Stimulator of interferon genes (STING) is an antiviral signalling protein that is broadly conserved in both innate immunity in animals and phage defence in prokaryotes. Here we use cryogenic electron microscopy to determine the structure of the active Toll/interleukin-1 receptor (TIR)–STING filament complex from a Sphingobacterium faecium cyclic-oligonucleotide-based antiphage signalling system (CBASS) defence operon. To define the molecular basis of STING filament formation, we reconstituted signalling of the S. faecium TIR–STING (SfSTING) antiphage effector in vitro and used single-particle cryo-EM to determine the structure of the activated complex. In each SfSTING dimer unit, the canonical V-shaped STING CBD is positioned above two TIR enzymatic NADase domains that dock against the base of the receptor.

The partially closed 3′,3′-cGAMP-bound SfSTING conformation allows incomplete oligomerization and is incompatible with stable filamentous packing beyond about 4–6 units (or about 20 nm). Compared to the fully active SfSTING–c-di-GMP filament structure, 3′,3′-cGAMP recognition induces partial closure of the lid domain and an overall conformation of the STING CDN-binding domain (CBD) that probably weakens contact sites observed for c-di-GMP-induced filaments. Additionally, a lack of well-defined density for the TIR domains in the 3′,3′-cGAMP filaments suggests conformational flexibility that may impact stability of the filaments. Our previous results demonstrate that 3′,3′-cGAMP binds with slightly weaker affinity (about 700 nM Kd) and is unable to induce robust TIR NADase activity, findings that are now explained by our cryo-EM analysis. Compared with the modelled open apo state and partially closed 3′,3′-cGAMP-bound conformations, recognition of the signal from the correct nucleotide, c-di-GMP, induces an inward rotation of the SfSTING β-strand ‘lid’ region of about 25° and about 9° respectively and results in formation of a tightly closed complex.

>MHHHHHHGSKKRIFIGSSSEQLTILNEIVDLLGDDVECIPWTDAFALNKSGLDSLIKQTRLADYSILIATKDDLTKQRGESLTKPRDNVVFEFGLFLGAAGPEKCYLIAEEDTDLPTDLDGITVAKFTRNSGQYNSLDKIVESIRTHLVKIAEMSQLGLLPSTALAIGYYNSFIKRVCEEIHGSECVELEGKKIKVKSFRVDVVIPETLDDNGVGNFTTLYNKRYGLSKATTCTNPALLGTRGFPFHFKVDPPDANQESPVDIHLLDIPSTLSTIVESLKLYLPSNQVGQDFDMDYLEMRELENFAKVLKYLIGRNAATKGYVNVLTNVKL[8x]>[2x]MLGTGPAAATTAATTSXXXXXXXXXXXXXXSRNEETXXXXXXXXXXXXXXXXXEMSQEEXTRFYDQLNHHIFELVSSSDANERKGGILAIASLIGVEGGNATRIGRFANYLRNLLPSNDPVVMEMASKAIGRLAMAGDTFTAEYVEFEVKRALEWLGADRNEGRRHAAVLVLRELAISVPTFFFQQVQPFFDNIFVAVWDPKQAIREGAVAALRACLILTTQREPKEMQKPQWYRHTFEEAEKGFDETLAKEKGMNRDDRIHGALLILNELVRISSMEGERLREEMEEITQQQLVHDKYCKDLMGFGTKPRHITPFTSFQAVQPQQSNALVGLLGYSSHQGLMGFGTSPSPAKSTXXXXXXXXXXXXXXXXXXXXXXXXXRNSKNSLIQMTILNLLPRLAAFRPSAFTDTQYLQDTMNHVLSCVKKEKERTAAFQALGLLSVAVRSEFKVYLPRVLDIIRAALPPKDFAHKRQKAMQVDATVFTCISMLARAMGPGIQQDIKELLEPMLAVGLSPALTAVLYDLSRQIPQLKKDIQDGLLKMLSLVLMXKPLRHPGMPKGLAHQLASPGLTTLPEASXVGSITLALRTLGSFEFEGHSLTQFVRHCADHFLNSEHKEIRMEAARTCSRLLTPSIHLISGHAHVVSQTAVQVVADVLSKLLVVGITDPDPDIRYCVLASLDERFDAHLAQAENLQALFVALNDQVFEIRELAICTVGRLSSMNPAFVMPFLRKMLIQILTELEHSGIGRIKEQSARMLGHLVSNAPRLIRPYMEPILKALILKLKDPDPDPNPGVINNVLATIGELAQVSGLEMRKWVDELFIIIMDMLQDSSLLAKRQVALWTLGQLVASTGYVVEPYRKYPTLLEVLLNFLKTEQNQGTRREAIRVLGLLGALDPYKHKVNIGMIDQSRDASAVSLSESKSSQDSSDYSTSEMLVNMGNLPLDEFYPAVSMVALMRIFRDQSLSHHHTMVVQAITFIFKSLGLKCVQFLPQVMPTFLNVIRVCDGAIREFLFQQLGMLVSFVKSHIRPYMDEIVTLMREFWVMNTSIQSTIILLIEQIVVALGGEFKLYLPQLIPHMLRVFMHDNSPGRIVSIKLLAAIQLFGANLDDYLHLLLPPIVKLFDAPEAPLPSRKAALETVDRLTESLDFTDYASRIIHPIVRTLDQSPELRSTAMDTLSSLVFQLGKKYQIFIPMVNKVLVRHRINHQRYDVLICRIVKGYTLADEEEDPLIYQHRMLRSGQGDALASGPVETGPMKKLHVSTINLQKAWGAARRVSKDDWLEWLRRLSLELLKDSSSPSLRSCWALAQAYNPMARDLFNAAFVSCWSELNEDQQDELIRSIELALTSQDIAEVTQTLLNLAEFMEHSDKGPLPLRDDNGIVLLGERAAKCRAYAKALHYKELEFQKGPTPAILESLISINNKLQQPEAAAGVLEYAMKHFGELEIQATWYEKLHEWEDALVAYDKKMDTNKDD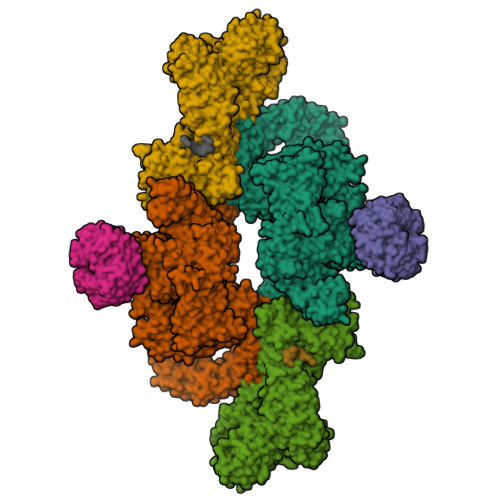PELMLGRMRCLEALGEWGQLHQQCCEKWTLVNDETQAKMARMAAAAAWGLGQWDSMEEYTCMIPRDTHDGAFYRAVLALHQDLFSLAQQCIDKARDLLDAELTAMAGESYSRAYGAMVSCHMLSELEEVIQYKLVPERREIIRQIWWERLQGCQRIVEDWQKILMVRSLVVSPHEDMRTWLKYASLCGKSGRLALAHKTLVLLLGVDPSRQLDHPLPTVHPQVTYAYMKNMWKSARKIDAFQHMQHFVQTMQQQAQHAIATEDQQHKQELHKLMARCFLKLGEWQLNLQGINESTIPKVLQYYSAATEHDRSWYKAWHAWAVMNFEAVLHYKHQNQARDEKKKLRHASGANITNATTAATTAATATTTASTEGSNSESEAESTENSPTPSPLQKKVTEDLSKTLLMYTVPAVQGFFRSISLSRGNNLQDTLRVLTLWFDYGHWPDVNEALVEGVKAIQIDTWLQVIPQLIARIDTPRPLVGRLIHQLLTDIGRYHPQALIYPLTVASKSTTTARHNAANKILKNMCEHSNTLVQQAMMVSEELIRVAILWHEMWHEGLEEASRLYFGERNVKGMFEVLEPLHAMMERGPQTLKETSFNQAYGRDLMEAQEWCRKYMKSGNVKDLTQAWDLYYHVFRRISKQLPQLTSLELQYVSPKLLMCRDLELAVPGTYDPNQPIIRIQSIAPSLQVITSKQRPRKLTLMGSNGHEFVFLLKGHEDLRQDERVMQLFGLVNTLLANDPTSLRKNLSIQRYAVIPLSTNSGLIGWVPHCDTLHALIRDYREKKKILLNIEHRIMLRMAPDYDHLTLMQKVEVFEHAVNNTAGDDLAKLLWLKSPSSEVWFDRRTNYTRSLAVMSMVGYILGLGDRHPSNLMLDRLSGKILHIDFGDCFEVAMTREKFPEKIPFRLTRMLTNAMEVTGLDGNYRITCHTVMEVLREHKDSVMAVLEAFVYDPLLNWRLMDTNTKGNKRSRTRTDSYSAGQSVEILDGVELGEPAHKKTGTTVPESIHSFIGDGLVKPEALNKKAIQIINRVRDKLTGRDFSHDDTLDVPTQVELLIKQATSHENLCQCYIGWCPFW;>MNTSPGTVGSDPVILATAGYDHTVRFWQAHSGICTRTVQHQDSQVNALEVTPDRSMIAAAGYQHIRMYDLNSNNPNPIISYDGVNKNIASVGFHEDGRWMYTGGEDCTARIWDLRSRNLQCQRIFQVNAPINCVCLHPNQAELIVGDQSGAIHIWDLKTDHNEQLIPEPEVSITSAHIDPDASYMAAVNSTGNCYVWNLTGGIGDEVTQLIPKTKIPAHTRYALQCRFSPDSTLLATCSADQTCKIWRTSNFSLMTELSIKSGNPGESSRGWMWGCAFSGDSQYIVTASSDNLARLWCVETGEIKREYGGHQKAVVCLAFNDSVLG[2x];>[2x]MDYKDDDDKESEMLQSPLLGLGEEDEADLTDWNLPLAFMKKRHCEKIEGSKSLAQSWRMKDRMKTVSVALVLCLNVGVDPPDVVKTTPCARLECWIDPLSMGPQKALETIGANLQKQYENWQPRARYKQSLDPTVDEVKKLCTSLRRNAKEERVLFHYNGHGVPRPTVNGEVWVFNKNYTQYIPLSIYDLQTWMGSPSIFVYDCSNAGLIVKSFKQFALQREQELEVAAINPNHPLAQMPLPPSMKNCIQLAACEATELLPMIPDLPADLFTSCLTTPIKIALRWFCMQKCVSLVPGVTLDLIEKIPGRLNDRRTPLGELNWIFTAITDTIAWNVLPRDLFQKLFRQDLLVASLFRNFLLAERIMRSYNCTPVSSPRLPPTYMHAMWQAWDLAVDICLSQLPTIIEEGTAFRHSPFFAEQLTAFQVWLTMGVENRNPPEQLPIVLQVLLSQVHRLRALDLLGRFLDLGPWAVSLALSVGIFPYVLKLLQSSARELRPLLVFIWAKILAVDSSCQADLVKDNGHKYFLSVLADPYMPAEHRTMTAFILAVIVNSYHTGQEACLQGNLIAICLEQLNDPHPLLRQWVAICLGRIWQNFDSARWCGVRDSAHEKLYSLLSDPIPEVRCAAVFALGTFVGNSAERTDHSTTIDHNVAMMLAQLVSDGSPMVRKELVVALSHLVVQYESNFCTVALQFIEEEKNYALPSPATTEGGSLTPVRDSPCTPRLRSVSSYGNIRAVATARSLNKSLQNLSLTEESGGAVAFSPGNLSTSSSASSTLGSPENEEHILSFETIDKMRRASSYSSLNSLIGVSFNSVYTQIWRVLLHLAADPYPEVSDVAMKVLNSIAYKATVNARPQRVLDTSSLTQSAPASPTNKGVHIHQAGGSPPASSTSSSSLTNDVAKQPVSRDLPSGRPGTTGPAGAQYTPHSHQFPRTRKMFDKGPEQTADDADDAAGHKSFISATVQTGFCDWSARYFAQPVMKIPEEHDLESQIRKEREWRFLRNSRVRRQAQQVIQKGITRLDDQIFLNRNPGVPSVVKFHPFTPCIAVADKDSICFWDWEKGEKLDYFHNGNPRYTRVTAMEYLNGQDCSLLLTATDDGAIRVWKNFADLEKNPEMVTAWQGLSDMLPTTRGAGMVVDWEQETGLLMSSGDVRIVRIWDTDREMKVQDIPTGADSCVTSLSCDSHRSLIVAGLGDGSIRVYDRRMALSECRVMTYREHTAWVVKASLQKRPDGHIVSVSVNGDVRIFDPRMPESVNVLQIVKGLTALDIHPQADLIACGSVNQFTAIYNSSGELINNIKYYDGFMGQRVGAISCLAFHPHWPHLAVGSNDYYISVYSVEKRVR;>[2x]GSGRMSGGSSCSQTPSRAIPATRRVVLGDGVQLPPGDYSTTPGGTLFSTTPGGTRIIYDRKFLMECRNSPVTKTPPRDLPTIPGVTSPSSDEPPMEASQSHLRNSPEDKRAGGEESQFEMDI>[2x]MRRREN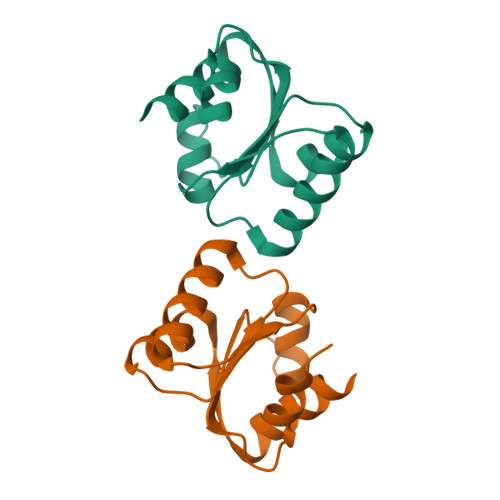MDVNKAIRTAVDTGKVILGSKRTIKFVKHGEGKLVVLAGNIPKDLEEDVKYYAKLSNIPVYQHKITSLELGAVCGKPFPVAALLVLDEGLSNIMELVEKKEGGE> GPDETLSLLADPYRFISRQCQRLGANAFESRFLLKKTNCLKGAKAAEIFYDTTRFEREGAMPVAIQKTLLGQGGVQGLDGETHRHRKQMFMGLMTPERVRALAQLFEAEWRRAVPGWTRKGEIVFYDELHEPLTRAVCAWAGVPLPDDEAGNRAGELRALFDAAGSASPRHLWSRLARRRVDAWAKRIIEGIRAGSIGSGSGTAAYAIAWHRDRHDDLLSPHVAAVELVNVLRPTVAIAVYITFVAHALQTCSGIRAALVQQPDYAELFVQEVRRFYPFFPAVVARASQDFEWEGMAFPEGRQVVLDL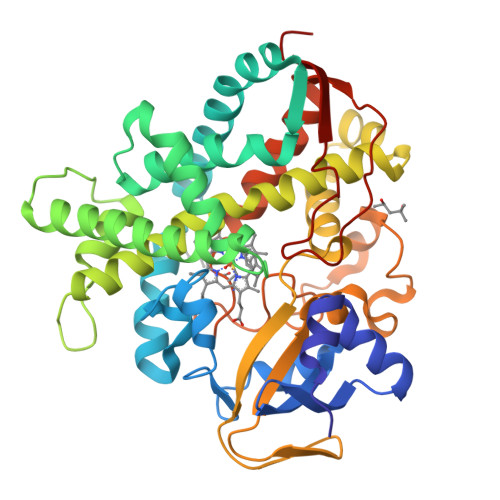YGSNHDAATWADPQEFRPERFRAWDEDSFNFIPQGGGDHYLGHRCPGEWIVLAIMKVAAHLLVNAMRYDVPDQDLSIDFARLPALPKSGFVMRNVHIGG> NSINDSKILSLQNKKNTLMDTSGYNAEVRVEGNVQLNPIFPFDFKLGSSGDDRGKVIVTQNENIVYNAMYESFSISFWIRINKWVSNLPG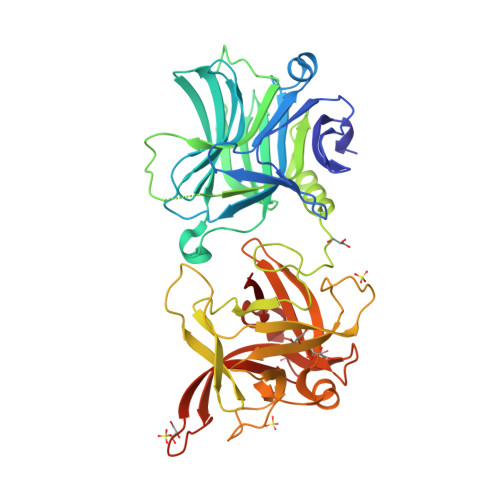YTIIDSVKNNSGWSIGIISNFLVFTLKQNENSEQDINFSYDISKNAAGYNKWFFVTITTNMMGNMMIYINGKLIDTIKVKELTGINFSKTITFQMNKIPNTGLITSDSDNINMWIRDFYIFAKELDDKDINILFNSLQYTNVVKDYWGNDLRYDKEYYMINVNYMNRYMSKKGNGIVFNTRKNNNDFNEGYKIIIKRIRGNTNDTRVRGENVLYFNTTIDNKQYSLGMYKPSRNLGTDLVPLGALDQPMDEIRKYGSFIIQPCNTFDYYASQLFLSSNATTNRLGILSIGSYSFKLGDDYWFNHEYLIPVIKIEHYASLLESTSTHWVFVPASE> MAQVQQLTPAQQAALRNQQAMAANLQARQIVLQQSYPVIQQVETQTFDPANRSVFDVTPANVGIVKGFLVKVTAAITNNHATEAVALTDFGPANLVQRVIYYDPDNQRHTETSGWHLHFVNTAKQGAPFLSSMVTDSPIKYGDVMNVIDAPATIAAGATGELTMYYWVPLAYSETDLTGAVLANVPQSKQRLKLEFANN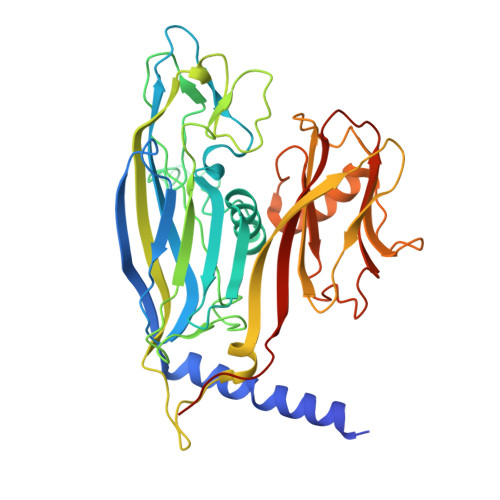NTAFAAVGANPLEAIYQGAGAADCEFEEISYTVYQSYLDQLPVGQNGYILPLIDLSTLYNLENSAQAGLTPNVDFVVQYANLYRYLSTIAVFDNGGSFNAGTDINYLSQRTANFSDTRKLDPKTWAAQTRRRIATDFPKGVYYCDNRDKPIYTLQYGNVGFVVNPKTVNQNARLLMGYEYFTSRTELVNAGTISTT> SRLSNAFVLATTASAAAVPSPALPADDILLAINQSLRLVDSRAAMLVSQVRHGAINNVGSLADSYHELIFS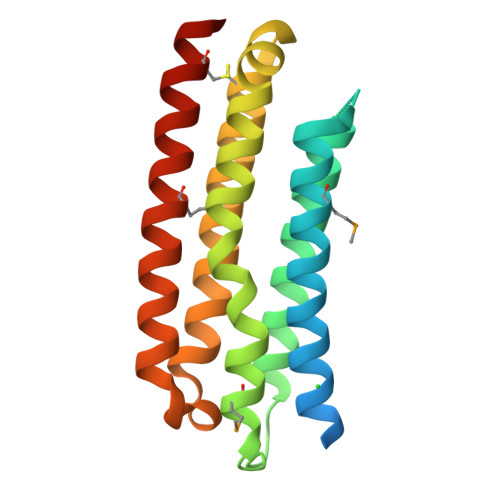LRGAVRAVDDVWRPLPKDAPMRIVESLRPFQKIPASLRSALKERLDAIAERPGGCQAVDDNNRQLGLDFDRLYWEIASSSSFSAIHETVSSQQKQFETAMRELTDEFSSRCLRRAQASA METHYL N-[(2S,3R)-3-AMINO-2-HYDROXY-3-(4-METHYLPHENYL)PROPANOYL]-D-ALANYL-D-LEUCINATE 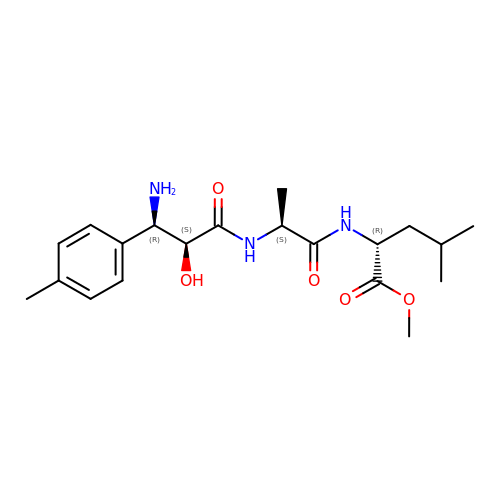| C20 H31 N3 O5 | BMHZOSJVDHAFEE-SVGFKBNWSA-N> ISIGYLLVKHSQTDQEPMCPVGMNKLWSGYSLLYFEGQEKAHNQDLGLAGSCLARFSTMPFLYCNPGDVCYYASRNDKSYWLSTTAPLPMMPVAEEDIRPYISRCSVCEAPAVAIAVHSQDVSIPHCPAGWRSLWIGYS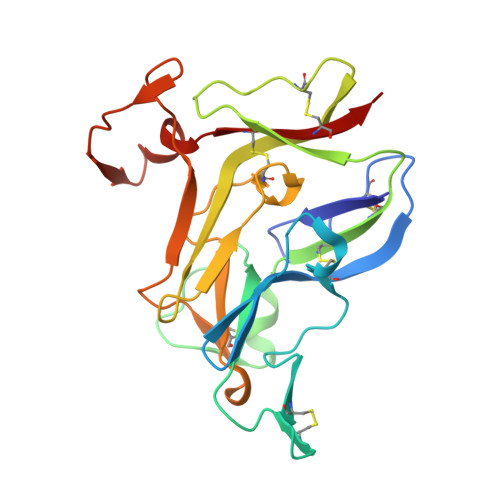FLMHTAAGDEGGGQSLVSPGSCLEDFRATPFIECNGARGTCHYYANKYSFWLTTIPEQSFQGTPSADTLKAGLIRTHISRCQVCMKNL In this study, we conducted the crystallization of a DNA/RNA heteroduplex in space and provide the first report on nucleic acid crystallization under microgravity and subsequent structure analyses. All of the crystals obtained both on Earth and in space belonged to space group P61, with almost identical unit-cell dimensions. All structures are similar to that determined in the previous study. Incidentally, spermine was observed due to the improved resolution in all four refined structures.

The lengths of the largest single crystal and the polycrystal were about 330 and 1260 µm, respectively. The maximum resolution determined according to the same criteria (the completeness is >99%; the Rmerge of the outer shell is around 35% or less; the multiplicity is about 5; the I/σ(I) in the outer shell is >3; the CC1/2 in the outer shell is >60%) was 1.5 Å for the Earth-1 crystal, 1.6 Å for the Space-1 crystal, 1.6 Å for the Earth-2 crystal and 1.4 Å for the Space-2 crystal. A comparison of the number of water molecules observed shows no notable differences: 97 in the previous study, 66 in the Earth-1 crystal, 53 in the Space-1 crystal, 76 in the Earth-2 crystal and 82 in the Space-2 crystal. The results showed no significant difference in the maximum resolution and crystal mosaicity between Earth and a microgravity environment. Therefore, the effect of the counter-diffusion method is likely to be more significant than the effect of microgravity in this study.

> GAAGAAGAG;> CTCTTCTTC> MADDVDNDDKLEKPVDLIWGCELNEQNKTFEFKVEDDEEKCEHQLALRTVCLGDKAKDEFHIVEIVDQEEGAEKVVPIATLKPSILPMATMVGIELDPPVTFRLKAGSGPLYISGQ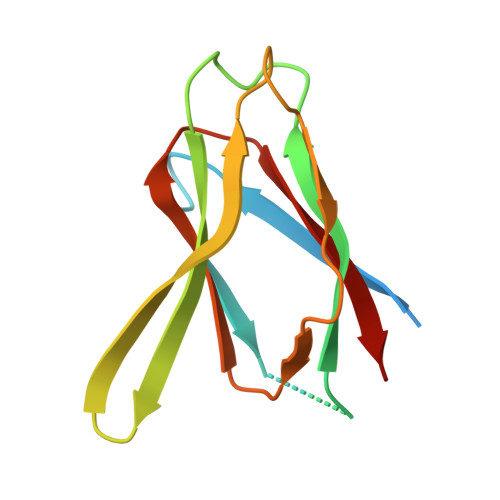HVAM> DDVSISPEQSFYEIMLIRPKTIDDINYVVDQVLEESNPVILDLSFLEKESPAN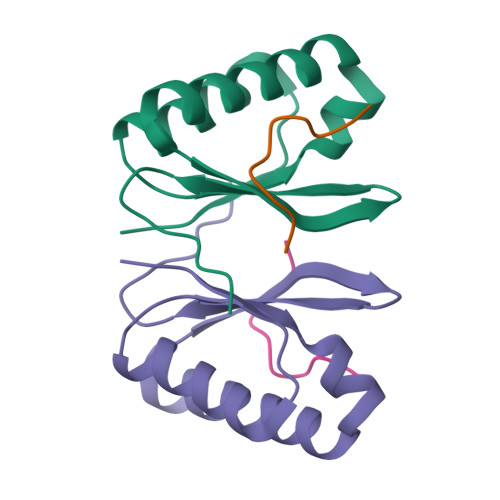FKLAGEKIKQMRSNYGAEALLLSRCNDKNLIIIAPKGVSLVRK;> QLDDFIDGIF> MATALYTANDFILISLPQNAQPVTAPGSKTDSWFNETLIGGRAFVSDFKIPEFKIGSLDTLIVESEELSKVDNQIGASIGKIIEILQGLNETSTNAYRTLPINNMPVPEYLENFQWQTRKFKLDKSIKDLITLISNESSQLDADVRATYANYNSAKTNLAAAERKKTGDLSVRSLHDIVKPEDFVLNSEHLTTVLVAVPKSLKSDFEKSYETLSKNVVPASASVIAEDAEYVLFNVHLFKKNVQEFTTAAREKKFIPREFNYSEELIDQLKKEHDSAAS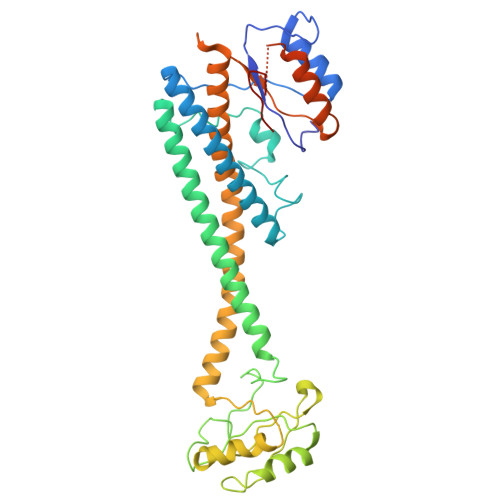LEQSLRVQLVRLAKTAYVDVFINWFHIKALRVYVESVLRYGLPPHFNIKIIAVPPKNLSKCKSELIDAFGFLGGNAFMKDKKGKINKQDTSLHQYASLVDTEYEPFVMYIINL>GIDPFTMASGSAGKPTGEAASPAPASAIGGASSQPRKRLVSVCDHCKGKMQLVADLLLLSSEARPVLFEGPASSGAGAESFEQCRDTIIARTKGLSILTHDVQSQLNMGRFGEAGDSLVELGDLVVSLTECSAHAAYLAAVATPGAQPAQPGLVDRYRVTRCRHEVEQGCAVLRATPLADMTPQLLLEVSQGLSRNLKFLTDACALASDKSRDRFSREQFKLGVKCMSTSASALLACVREVKVAPSELARSRCALF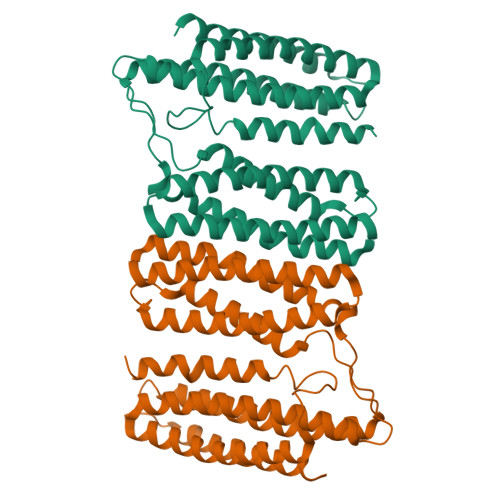SGPLVQAVSALVGFATEPQFLGRAAAVSAEGKAVQTAILGGAMSVVSACVLLTQCLRDLAQHPDGGAKMSDHRERLRNSACAVSEGCTLLSQALRERSSPRTLPPVNSNSVN[2x]>MNAEINPLHAYFKLPNTVSLVAGSSEGETPLNAFDGALLNAGIGNVNLIRIS[6x];>XIMPPEAEIVPLPKLPMG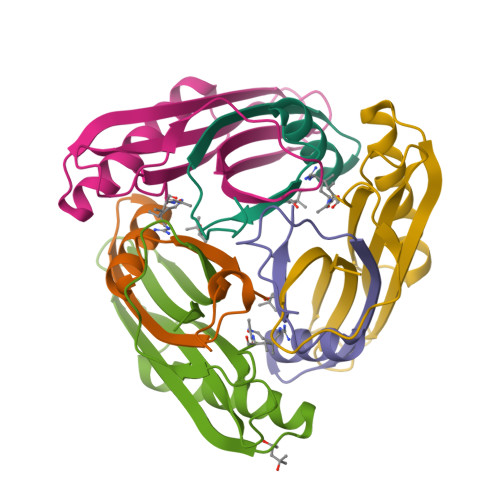ALVPTAYGYIISDVPGETISAAISVAIPKDKSLCGLIMEYEGKCSKKEAEKTVREMAKIGFEMRGWELDRIESIAVEHTVEKLGCAFAAAALWYK[6x]6-[(3S,4S)-4-methyl-1-(pyrimidin-2-ylmethyl)pyrrolidin-3-yl]-1-(tetrahydro-2H-pyran-4-yl)-1,5-dihydro-4H-pyrazolo[3,4-d]pyrimidin-4-one | 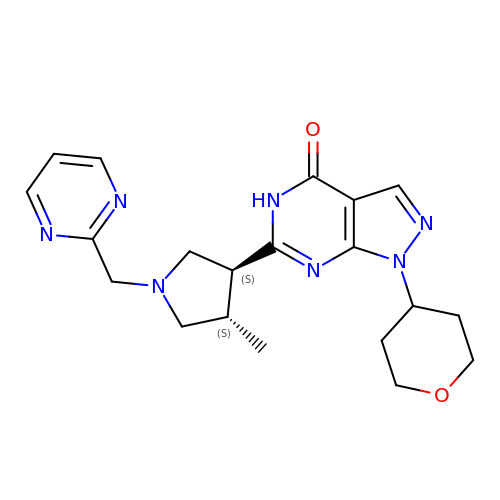C20 H25 N7 O2 | IWXUVYOOUMLUTQ-CZUORRHYSA-N>[2x]MALSQATDPFRAAVEFTLMPMLITNPHLPDNPIVFANPAFLKLTGYEADEVMGRNCRFLQGHGTDPAHVRAIKSAIAAEKPIDIDIINYKKSGEAFWNRLHISPVHNANGRLQHFVSSQLDVTLELSRLVELEKERKTLSIETARSKDQLDYIVEVANIGFWTREFYSGKMTCSA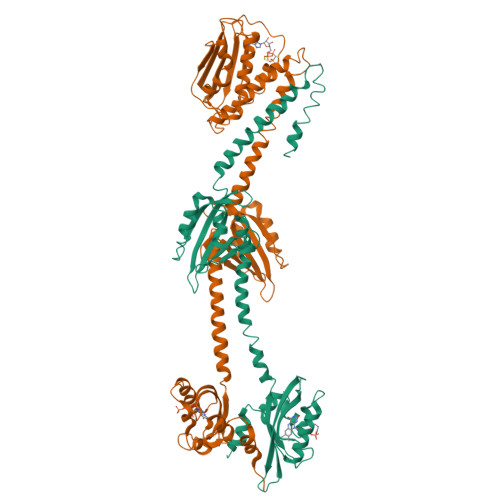ECRRIYGFTPDEPVHFDTILDLVVLEDRMTVVQKAHQAVTGEPYSIEYRIVTRLGETRWLETRAKALTGENPLVLGIVQDVTERKKAEANKALVSREIAHRFKNSMAMVQSIANQTLRNTYDPEQANRLFSERLRALSQAHDMLLKENWAGATIQQICATALAPFNSTFANRIHMSGPHLLVSDRVTVALSLAFYELATNAVKYGALSNEKGVINITWAIMEDKGEKKFHMRWAESRGPEVMQPARRGFGQRLLHSVLAEELKAKCDVEFAASGLLIDVLAPITPEVFPGMGHNVPEQRIAHHHHHH>[2x]MILIRGLTRVITFDDQERELEDADILIDGPKIVAVGKDLSDRSVSRTIDGRGMIALPGLINSHQHLYEGAMRAIPQLERVTMASWLEGVLTRSAGWWRDGKFGPDVIREVARAVLLESLLGGIT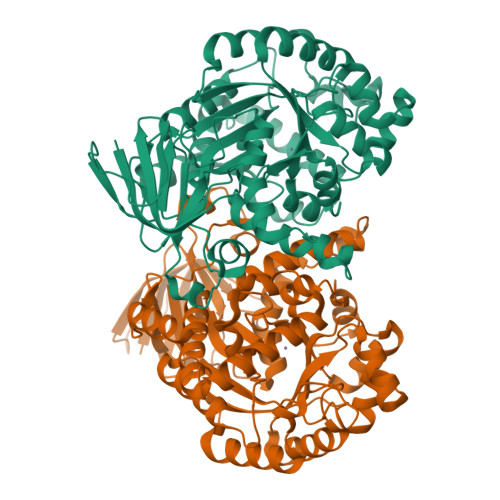TVADQHLFFPGATADSYIDATIEAATDLGIRFHAARSSMTLGKSEGGFCDDLFVEPVDRVVQHCLGLIDQYHEPEPFGMVRIALGPCGVPYDKPELFEAFAQMAADYDVRLHTHFYEPLDAGMSDHLYGMTPWRFLEKHGWASDRVWLAHAVVPPREEIPEFADAGVAIAHLIAPDLRMGWGLAPIREYLDAGITVGFGTTGSASNDGGNLLGDLRLAALAHRPADPNEPEKWLSARELLRMATRGSAECLGRPDLGVLEEGRAADIACWRLDGVDRVGVHDPAIGLIMTGLSDRASLVVVNGQVLVENERPVLADLERIVANTTALIPKNL>[8x]SNAKEPSCMSSIIPGWFSEISPMWPGEAHSLKVEKILFQGKSDYQDVIVFQSATYGKVLVLDGVIQLTERDECAYQEMITHLPLCSISNPKKVLVIGGGDGGVLREVARHSSVEQIDICEIDKMVVDVAKQYFPNVAVGYEDPRVNLIIGDGVAFLKNAAEGTYDAVIVDSSDPIGPAKELFEKPFFESVNRALRPGGVVCTQAESLWLHMDIIEDIVSNCRD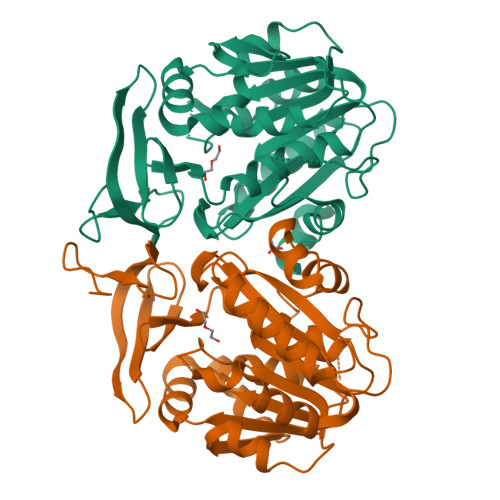IFKGSVNYAWTSVPTYPSGVIGFMLCSSEGPQVDFKKPVSLIDTDESSIKSHCPLKYYNAEIHSAAFCLPSFAKKVIDSKAN>AVPKIRIAVPSKGRISEPAIRLLENAGVGLKDTVNRKLFSKTQHPQIEVMFSRAADIPEFVADGAADLGITGYDLIVERGSDVEILEDLKYGRASLVLAAPEDSTIRGPEDIPRGAVIATEFPGITENYLREHGIDAEVVELTGSTEIAPFIGVADLITDLSSTGTTLRMNHLRVIDTILESSVKLIANRESY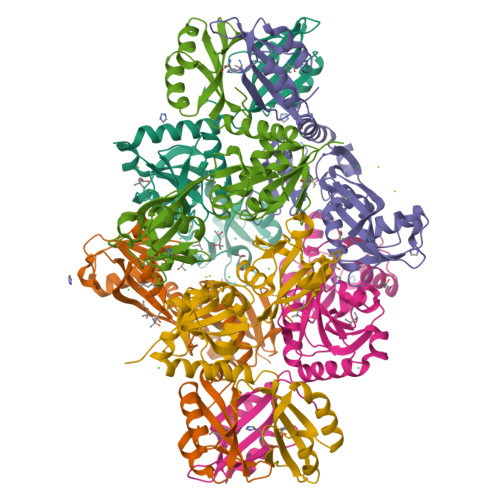ATKSGIIEELRTGIRGVIDAEGKRLVMLNIDRKNLDRVRALMPGMTGPTVSEVLSDNGVVAVHAVVDEKEVFNLINRLKAVGARDILVVPIERIIP[2x]>[3x]MAKLLIMSIVSFCFIFLLLLFFRYILKRYFNYMLNYKVWYLTLLAGLIPFIPIKFSLFKFNNVNNQAPTVESKSHDLNHNINTTKPIQEFATDIHKFNWDSIDNICTVIWIVLVIILSFKFLKALLYLKYLKKQSLYLNENEKNKIDTILFNHQYKKNIVIRKAETIQSPITFWYGKYIILIPSSYFKSVIDKRLKYIILHEYAHAKNRDTLHLIIFNIFSIIMSYNPLVHIVKRKIIHDNEVEADRFVLNNINKNEFKTYA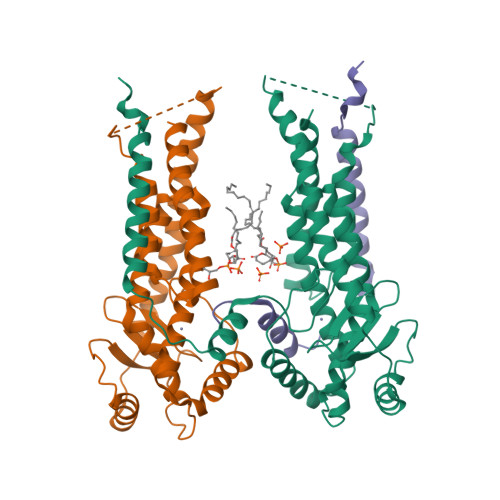ESIMDSVLNVPFFNKNILSHSFNGKKSLLKRRLINIKEANLKKQSKLILIFICIFTFLLMVIQSQFLMGQSITDYNYKKPLHNDYQILDKSKIFGSNSGSFVMYSMKKDKYYIYNEKESRKRYSPNSTYKIYLAMFGLDRHIINDENSRMSWNHKHYPFDAWNKEQDLNTAMQNSVNWYFERISDQIPKNYTATQLKQLNYGNKNLGSYKSYWMEDSLKISNLEQVIVFKNMMEQNNHFSKKAKNQLSSSLLIKKNEKYELYGKTGTGIVNGKYNNGWFVGYVITNHDKYYFATHLSDGKPSGKNAELISEKILKEMGVLNGQELALVPRGSSAHHHHHH>[4x]GSEFEPVSKLRIRTPSGEFLERRFL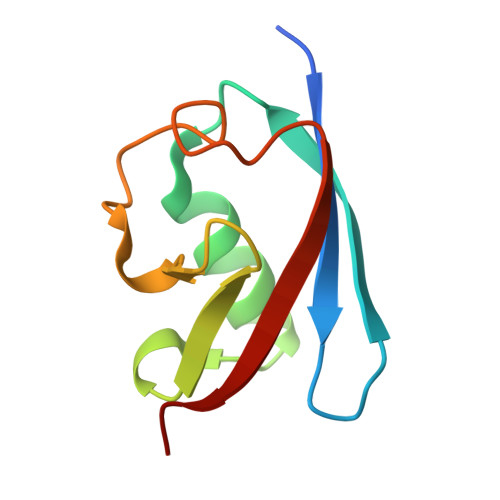ASNKLQIVFDFVASKGFPWDEYKLLSTFPRRDVTQLDPNKSLLEVKLFPQETLFLEAKE>[3x]SKKTVEFVDYVNPLMGTESTFAFSHGNTYPAVAVPWGMNFWSPQTGENGSGWMYTYTDSLMRGFRQTHQPSPWINDYGTFSIMPLAGELKMSHKERLVPFSHQQEKATPYNYSVTFNNGLQTSLSATSRGAVFEVSFPEKEDQYVVVDAYN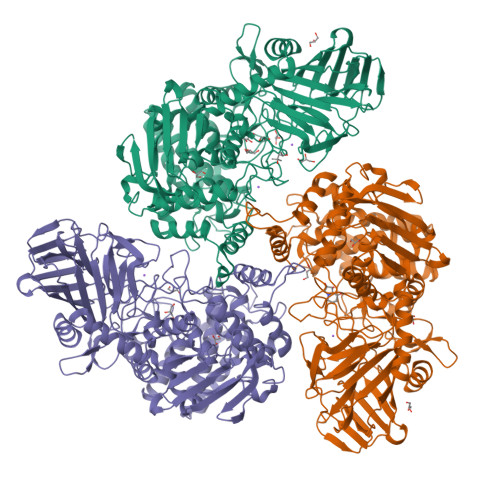GGSSITIEPEKRLVKGATRYNNGGVPDNFANYFMMEFSHPVIEYGTYNGDTLLHHQTDVAADYTCAYLKFDVPAGEKLTIRTASSFISPEQAAINFNREVADADVQLISGKAREQWNNYLGRVEAEGGTDEQLRTFYSCLYRTLLFPREFYEFDSQGNPVYYSPYDGNVHDGYMYTDNGFWDTFRAVHPLFTLLYPEVSERVTQSIINAYNESGFMPEWASPGHRGCMIGNNSVSLLVDAWMKGIQTVDAEKALEAMIHQTQARHAEIASVGRDGFEYYDKLGYVPYPEVPEATAKTLEYAYADWCIARFAESLGKQDIADQYYQKAPNYRNLYYPEHGFMWTKDAKGNWRDRFDATEWGGPFTEGSSWHWTWSVFHDPEGLSELMGGHEPMIARLDSMFVAPNTYNYGTYGFVIHEIAEMVALNMGQYAHGNQPVQHAIYLYDYIGQPWKTQYHLRNVMDKLYNSGSKGYCGDEDNGQTSAWYVFSAMGFYPVCPGMPEYAIGSPLFKKVTLHLPEGKNFVVSAADNAADRPYIRKALLNGQEFTRNYLTHDELKQGGELNLSMDSVPNQQRGTQPADFPYSYSK N-(5-(4-CHLORO-3-(2-HYDROXY-ETHYLSULFAMOYL)- 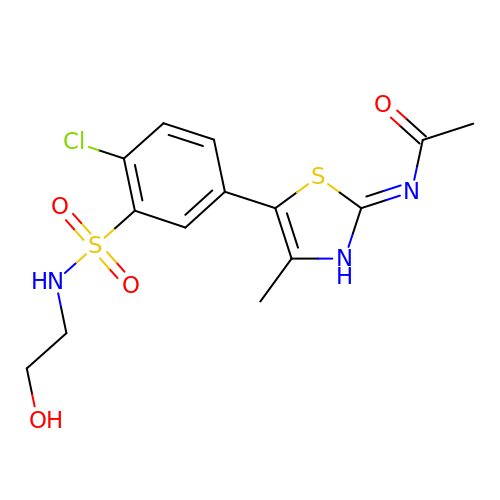PHENYLTHIAZOLE-2-YL)-ACETAMIDE | C14 H16 Cl N3 O4 S2 | JFVNFXCESCXMBC-UHFFFAOYSA-N> NATEIRASVGKMIDGIGRFYIQMCTELKLSDYEGRLIQNSLTIERMVLSAFDTGGPIYRRVDGKWRRELILYDKEEIRRIWRQANNGDDATAGLTHMMIWHSNLNDATYQRTRALVRTGMDPRMCSLMQGSTLPRRSGA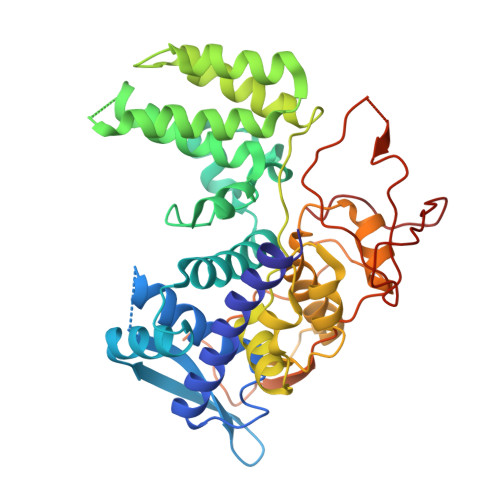AGAAVKGVGTMVMELIRMIKRGINRRTRIAYERMCNILKGKFQTAAQRTMVDQVRESRNPGNAEFEDLIFLARSALILRGSVAHKSCLPACVYGSAVASGYDFEREGYSLVGIDPFRLLQNSQVYSLIRPNENPAHKSQLVWMACHSAAFEDLRVSSFIRGTKVVPRGKLSTRGVQIASNENMETMESSTLELRSRYWAIRTRSGGNTDVSFQGRGVFELSDEKATSPIVPSFDMSNEGSYFF>[2x]MKVGIDAGGTLIKIVQEQDNQRTFKTELTKNIDQVVEWLN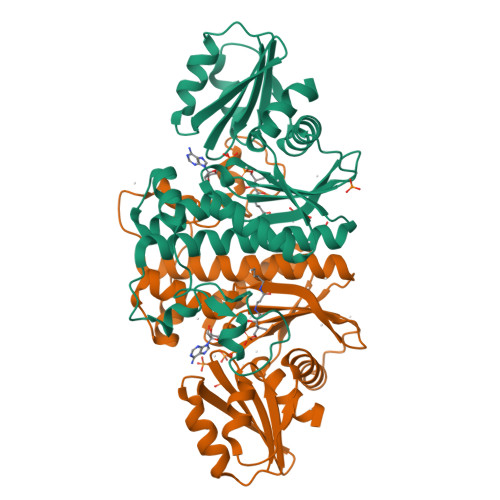QQQIEKLCLTGGNAGVIAENINIPAQIFVEFDAASQGLGILLKEQGHDLADYIFANVGTGTSLHYFDGQSQRRVGGIGTGGGMIQGLGYLLSQITDYKQLTDMAQHGDRNTIDLKVRHIYKDTEPPIPGDLTAANFGHVLHHLDADFTPSNKLAAVIGVVGEVVTTMAITVAREFKTENIVYIGSSFHNNALLRKVVEDYTVLRGCKPYYVENGAFSGAIGALYLEKHHHHHH>GPAMFEARLVQGSILKKVLEALKDLINEACWDISSSGVNLQSMDSSHVSLVQLTLRSEGFDTYRCDRNLAMGVNLTSMSKILKCAGNEDIITLRAEDNADTLALVFEAPNQEKVSDYEMKLMDLDVEQLGIPEQEYSCVVKMPSGEFARICRDLSHIGDAVVISCAKDGVKFSASGELGNGNIKLSQTSNVDKEEEAVTIEMNEPVQLTFALRYLNFFTKATPLSSTVTLSMSADVPLVVEYKIADMGHLKYYLAPKIEDEEGS[6x];>QHGKK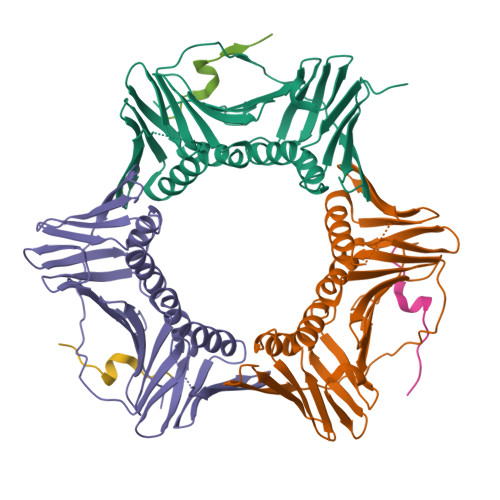DSKITDHFMRLPKA[6x]>GLHALMTAEELAFFARFGRMREIAAGQALFERGAVGTQMFIVVTGQIDLDFGEDLMLKHLGPGEFFGELGLLIGDHARSAGASASVDSRLIELAHDDFQRLVDHDPSMVAHFLRRSIVRVVNNEQLLIR[2x]

One candidate cyclic GMP effector is XC_0249, a protein with a predicted cyclic mononucleotide-binding (cNMP) domain attached to a GGDEF domain that is active in synthesis of cyclic di-GMP. Our data suggest that the action of cyclic GMP in Xcc depends in part on XC_0249, which has a cyclic GMP-binding domain attached to a GGDEF domain active in cyclic di-GMP synthesis. The findings showed that cyclic GMP addition led to an increase in the activity of XC_0249 in cyclic di-GMP synthesis. Mutation of either XC_0250 or XC_0249 led to a reduced virulence to plants and reduced biofilm formation in vitro. These findings describe a regulatory pathway in which cyclic GMP regulates virulence and biofilm formation through interaction with a novel effector that directly links cyclic GMP and cyclic di-GMP signalling.

To further characterise the binding of cyclic GMP by the cNMP domain of XC_0249, we determined the crystal structure of the domain with the nucleotide bound to a resolution of 2.2 Å. The XC_0249 cyclic NMP-binding domain crystallises as a dimer. The Fo-Fc electron density map of the complex showed a clear electron density for cyclic GMP adopting a syn configuration when bound to the protein, that is with the ribose H1’ and guanine H8 bonds oriented in the same direction. Cyclic GMP makes a number of contacts with the residues surrounding the ligand-binding pocket. A number of these residues form specific H bonds with the ribose 2′-OH, phosphate lactone oxygen atoms and, importantly, with the guanine base. Residue E146 is especially interesting, as it is located within the opposing αC helix, with its two carboxylate oxygen atoms forming two crucial H bonds with the guanine N1 and N2 atoms. N145 is also a critical residue, as its side chain amide nitrogen atom forms one H bond with the guanine O6 atom. In addition, potential hydrophobic interactions are also involved in cyclic GMP binding; F73 is involved in a perpendicular C–H bond/purine base interaction, and L91 and V142 are involved in interactions at the other face of the ligand with the ribose and guanine base. The XC_0249 cyclic NMP domain dimer exhibits an interface area of 1344 Å2, and each cyclic GMP exhibits an interface area of ∼300 Å2, giving a ΔG of −2.9 kcal mol−1 as calculated using the PISA program. The major difference between the two structures is the diad motif of N145 and E146, which form strong H bonds with the guanine base of cyclic GMP and which contribute to cyclic GMP binding.3-OXO-OCTANOIC ACID (2-OXO-TETRAHYDRO-FURAN-3-YL)-AMIDE 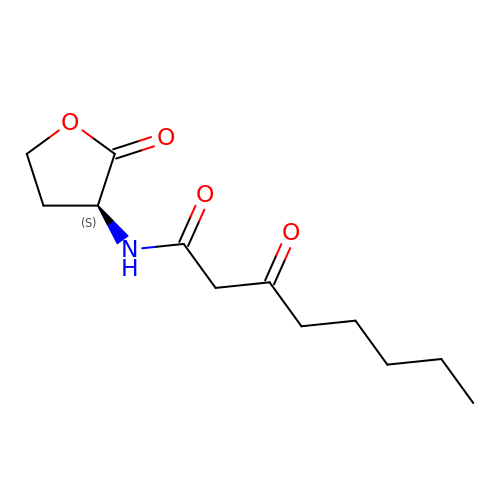| C12 H19 N O4 | FXCMGCFNLNFLSH-JTQLQIEISA-N>[2x]MSRLVLLVNPNKVHPPIAPYALDVLTTALEDEGFEVEVLDLTFRRDDWKTCLHEYFAERSPMLVGVTVRNTDTVYAFEQRPFVGEHREIITEIRRLTDAPVVGGGIGFSTMPFALVEYFGIEYGVKGPGEKILCELATAISEGRDTAGIPGLIRNTERGAVRVPPAVLTVRHGKTQPAEPTGQFEPRVWQVDQLSVYRRRSGVPRKVDNLEYYRRGGLGSILTKNGCAYRCSHCVEPDAKGTRYGQRELASVVDEMESLAAQGILDQHTTDSEFNLSIAHAKNLLREIVRRRHADPDNPLNRLRLWVYCQPSPFDEEF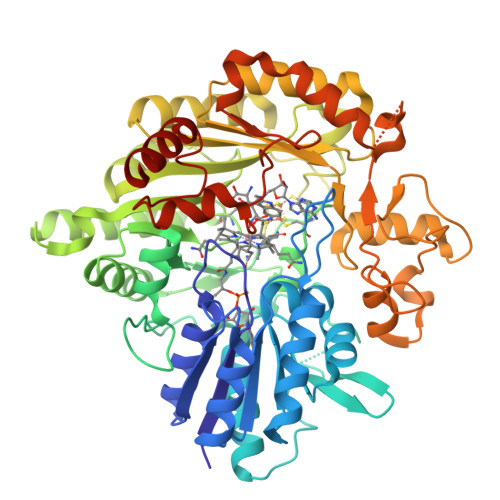ADLLAAAGCRGVNVGSDHIRPELLSGWKVTEKGGTYYTFEDTERLVRLCRERGILTMVEALFGMPGETPETVRACVDAFMALDATVTGFSLGLRLFPYTPMGIEIAEQCAGVRTAPGLQSNTADGPIVLKPLRMCASPAEYERQFMFDEHGNFRLVCYFSPGLLPDPARAADPEERWHGAVADLWALIDPADHHRVMLPTVEGMSEHDNNYADNPFLTSLGGLGYTGAFWSHWRGREEIMRKAREAAAQSSHLPTPV> MMPDDNSNSSTQNSSALYKDLRKEYESLFTLKEDSGLEISPIFNVLPPKKDYPDYYAVIKNPVSFNTLKKRIPHYTDAQQFMNDVVQIPWNAKTYNTRDSGIYKYALVLEKYLKDTIYPNLKEKYPQLVYPDLGPLPDEPGYEEFQQKLREKAEEVARANAARAESSSSMN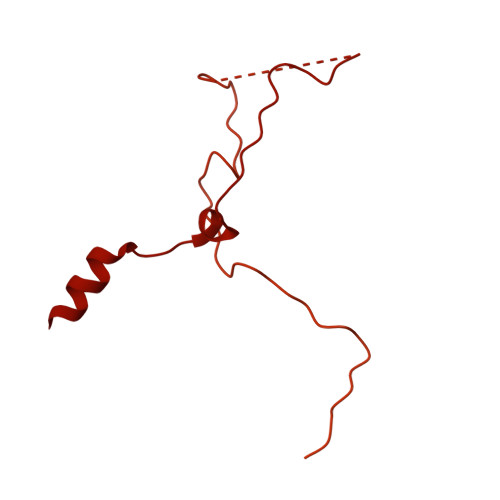STEAARRLRKTRTSVKRESEPGTDTNNDEDYEATDMDIDNPKDADFPDLIRKPLININPYTRKPLRDNRSTTPSHSGTPQPLGPRHRQVSRTQVKRGRPPIIDLPYIQRMKNVMKVLKKEVLDSGIGLTDLFERLPDRHRDANYYIMIANPISLQDINKKVKTRRYKTFQEFQNDFNLMLTNFRISHRGDPESIKISNILEKTFTSLARFELSKPDRSFIPEGELRYPLDEVIVNNISYHVGDWALLRNQNDPQKPIVGQIFRLWKTPDGKQWLNACWYYRPEQTVHRVDRLFYKNEVMKTGQYRDHLVSNLVGKCYVIHFTRYQRGNPDMKLEGPLFVCEFRYNESDKIFNKIRTWKACLPEEIRDLDEATIPVNGRKFFKYPSPIRHLLPANATPHDRVPEPTMGSPDAPPLVGAVYMRPKMQRDDLGEYATSDDCPRYIIRPNDSPEEGQVDIETGTITTNTPTANALPKTGYSSSKLSSLRYNRSSMSLENQNAIGQQQIPLSRVGSPGAGGPLTVQGLKQHQLQRLQQQQHQYQQQKRSQASRYNIPTIIDDLTSQASRGNLGNIMIDAASSFVLPISITKNVDVLQRTDLHSQTKRSGREEMFPWKKTKGEILWFRGPSVIVNERIINSGDPHLSLPLNRWFTTNKKRKLEYEEVEETMEDVTGKDKDDDGLEPDVENEKESLPGPFVLGLRPSAKFTAHRLSMLRPPSSSS> MVYSYTEKKRIRKDFGKRPQVLDVPYLLSIQLDSFQKFIEQDPEGQYGLEAAFRSVFPIQSYSGNSELQYVSYRLGEPVFDVQECQIRGVTYSAPLRVKLRLVIYEREAPEGTVKDIKEQEVYMGEIPLMTDNGTFVINGTERVIVSQLHRSPGVFFDSDKGKTHSSGKVL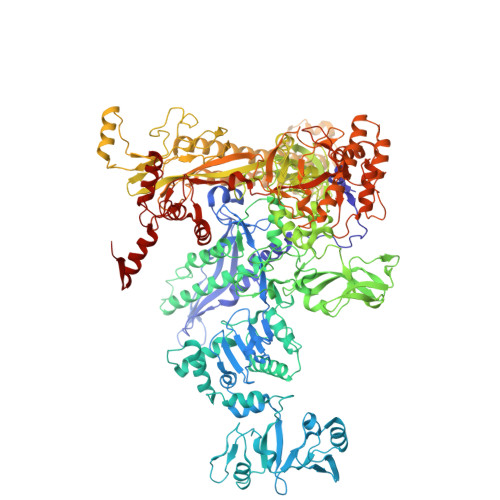YNARIIPYRGSWLDFEFDPKDNLFVRIDRRRKLPATIILRALNYTTEQILDLFFEKVIFEIRDNKLQMELVPERLRGETASFDIEANGKVYVEKGRRITARHIRQLEKDDVKLIEVPVEYIAGKVVAKDYIDESTGELICAANMELSLDLLAKLSQSGHKRIETLFTNDLDHGPYISETLRVDPTNDRLSALVEIYRMMRPGEPPTREAAESLFENLFFSEDRYDLSAVGRMKFNRSLLREEIEGSGILSKDDIIDVMKKLIDIRNGKGEVDDIDHLGNRRIRSVGEMAENQFRVGLVRVERAVKERLSLGDLDTLMPQDMINAKPISAAVKEFFGSSQLSQFMDQNNPLSEITYKRRISALGPGGLTRERAGFEVRDVHPTHYGRVCPIETPEGPNIGLINSLSVYAQTNEYGFLETPYRKVTDGVVTDEIHYLSAIEEGNYVIAQANSNLDEEGHFVEDLVTCRSKGESSLFSRDQVDYMDVSTQQVVSVGASLIPFLEHDDANRALMGANMQRQAVPTLRADKPLVGTGMERAVAVDSGVTAVAKRGGVVQYVDASRIVIKVNEDEMYPGEAGIDIYNLTKYTRSNQNTCINQMPCVSLGEPVERGDVLADGPSTDLGELALGQNMRVAFMPWNGYNFEDSILVSERVVQEDRFTTIHIQELACVSRDTKLGPEEITADIPNVGEAALSKLDESGIVYIGAEVTGGDILVGKVTPKGETQLTPEEKLLRAIFGEKASDVKDSSLRVPNGVSGTVIDVQVFTRDGVEKDKRALEIEEMQLKQAKKDLSEELQILEAGLFSRIRAVLVAGGVEAEKLDKLPRDRWLELGLTDEEKQNQLEQLAEQYDELKHEFEKKLEAKRRKITQGDDLAPGVLKIVKVYLAVKRRIQPGDKMAGRHGNKGVISKINPIEDMPYDENGTPVDIVLNPLGVPSRMNIGQILETHLGMAAKGIGDKINAMLKQQQEVAKLREFIQRAYDLGADVRQKVDLSTFSDEEVMRLAENLRKGMPIATPVFDGAKEAEIKELLKLGDLPTSGQIRLYDGRTGEQFERPVTVGYMYMLKLNHLVDDKMHARSTGSYSLVTQQPLGGKAQFGGQRFGEMEVWALEAYGAAYTLQEMLTVKSDDVNGRTKMYKNIVDGNHQMEPGMPESFNVLLKEIRSLGINIELEDE>MAHHHHHHMQVYHLSHIDLDGYACQLVSKQFFKNI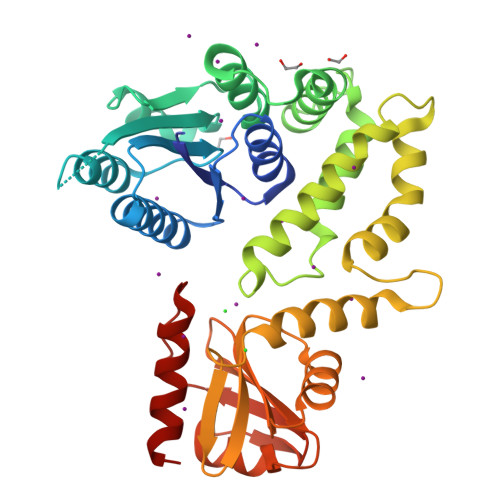QCYNANYGREVSARIYEILNAIAQSKESEFLILVSDLNLNLNEAEYLQDKIQEHRLQNKNIQIQLLDHHISGKEVAESFHWYFLDTNRCATKIVYEFLKKHYAILEPKNTTWLEPLVEMVNSVDIWDTQGYGFELGKVCMRMITQSSELNRFMFDDENRDYKLKLLEEVKNYLFLENAPVAYDNDLFRLKKIALGGDPDTETMDNISSNAQTHLLSLKKHDCSVYYQDKKGFLSYSMGGISVLANLFLTQNPDFDFYIDVNAKGNVSLRANGNCDVCELSQMCFNGGGHRNASGGKIDGFRESFNYRDIKEQIEEIFNNA[2x]>[6x]MSGSHHHHHHSGSMSERPSDLVVNRLVLFVVKGTATSTHNTVKPLILLEELGVPHDIYVVEKVSAPWFSEINPHKMVPAILDRSPDGRDTLRAWQSTSTLMYIADAYDKDGT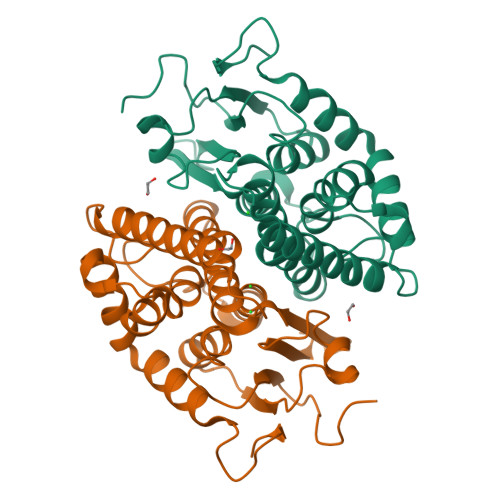FGGRNVQERSEINNWLTLHTAALGPTAKYWLYFYKLHPEKLPKTIEKLRSNITVQYDILERRLNEPGQQYLALKDRPTIADIATLPFAMKSTAELFGLEFEKWPKLQEWSVRMGEREAVKRAWQRVAGFGHGEKEYGMLEA> MTTNSSSNTVVVYHSGYGHTHRMAEAVAEGAEATLHAIDAEGNLSEDGWAALDAADAIIFGTPTY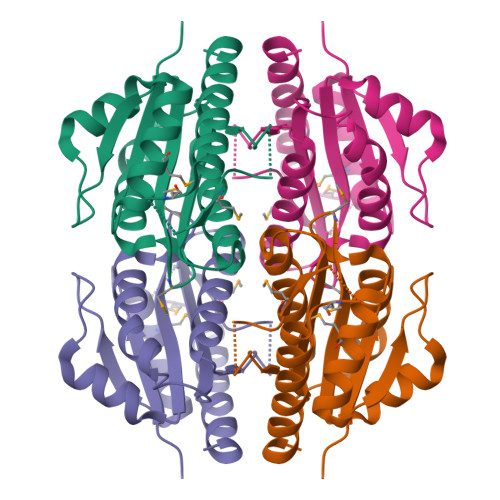MGGPSWQFKKFADASSKPWFSAKWQDKVFGGFTNSASLNGDKLNTLQYLVLLAGQHGGLWVSLGIKPSNLKSSVRNDANRMGSYIAPMAQSDADAAPEEMSVGDLETARLYGARVANVARQHKSTERV During biosynthesis by multi-modular trans-AT polyketide synthases, polyketide structural space can be expanded by conversion of initially-formed electrophilic β-ketones into β-alkyl groups. These multi-step transformations are catalysed by 3-hydroxy-3-methylgluratryl synthase cassettes of enzymes. In this work, we investigated the β-methylation module 5 present in the virginiamycin (Vir) trans-AT PKS-NRPS, which comprises a KS domain and tandem ACPs (ACP5a and ACP5b). We show here that β-methylation cassette members VirC, VirD and VirE do indeed preferentially recognise ACP5b, even when the ACP is excised from its modular context, and that β-modification occurs within defined ACP5b/partner complexes.

The final VirD model consists of a trimer in the asymmetric unit with r.m.s.d. between monomers of 0.2 Å (202 Cα), whose solution relevance was confirmed by SAXS analysis (CRYSOL21). Notably, the interface also incorporates the well-folded helix α10 of the first monomer, which is disordered in the structure of VirD alone.

>[3x]GPGSVRVVRGRGLLRAVLDRPERRNPIDAGLLTSLARALDQAESDQDCRVFVLSSTGEDFCAGTDLSGGDPAPEPLPDGAELPYWTLLERLTRSPLATVAVVDGRATAGGVGLAAACDLVLAGERARFRLTEVLAGLVPAMALPFVARRTGEQRAFAATLRAEEFDAGAAHRVGLADLAGPRAEDLLPPVLAGLGRTDRSTTAALKEYRARLFPRDARLGHDASRLLIERFAAPGTGQLLARLREAGAAA> MDLSELERDNTGRCRLSSPVPAVCLKEPCVLGVDEAGRGPVLGPMVYAICYCPLSRLADLEALKVADSKTLTENERERLFAKMEEDGDFVGWALDVLSPNLISTSMLGRVKYNLNSLSHDTAAGLIQYALDQNVNVTQVFVDTVGMPETYQARLQQHFPGIEVTVKAKADSLFPVVSAASIFAKVARDKAVKNWQFVENLQDLDSDYGSGYPNDPKTKAWLRKHVDPVFGFPQFVRFSWSTAQAILEKEAED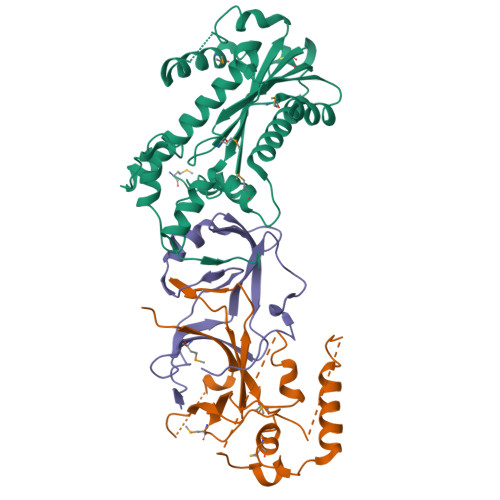VIWEDSEAEEDPERPGKITSYFSQGPQTCRPQAPHRYFQERGLEAASSL;> MGSSHHHHHHSQDPNSLEVLFQGPMAGGRDRGDLAARQLVFLLPEHLKDASKKKKKSSLLFVKLANPHSGEGATYLIDMCLQQLFEIKVFKEKHHSWFINQSVQSGGLLHFATPMDPLFLLLHYLLKAGKEGKYQPLDQVVVDDTFPDCTLLLRFPELEKSLRHVTEEKEVNSKKYYKYSSEKTLKWLEKKVNQTVVALKANNVNVGARVQSSAYFSGGQVSRDKEEDYVRYAHGLISDYIPKELSDDLSKFLKLPEPPASLPNPPSKKLKLSDEPVEAKEDYTKFNTKDLKTGKKNSKMTAAQKALAKVDKSGMKSIDAFFGAKNKKTGKI;> MKNPEEAAEGKQRIHLRPGSLRGAAPAKLHLLPCDVLVSRPAPVDRFFTPAVRHDADGLQASFRGRGLRGEEVAVPPGFAGFVMVTEEKGEGLIGKLNFSGDAEDKADEAQEPLERDFDRLIGATGSFSHFTLWGLETVPGPDAKVHRALGWPSLAAAIHAQVPED>[2x]YSGPKLEDGKVTISFMKELMQWYKDQKKLHRKCAYQILVQVKEVLSKLSTLVETTLKETEKITVCGDTHGQFYD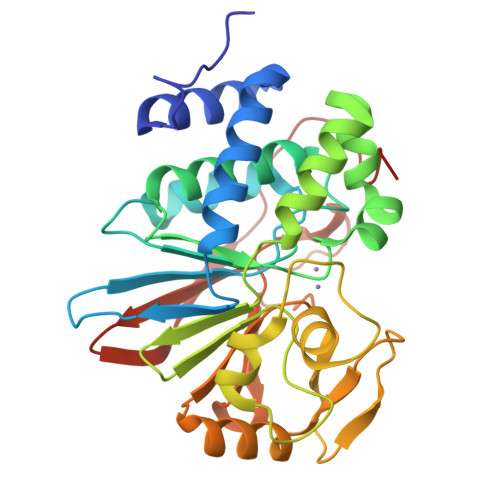LLNIFELNGLPSETNPYIFNGDFVDRGSFSVEVILTLFGFKLLYPDHFHLLRGNHETDNMNQIYGFEGEVKAKYTAQMYELFSEVFEWLPLAQCINGKVLIMHGGLFSEDGVTLDDIRKIERNRQPPDSGPMCDLLWSDPQPQNGRSISKRGVSCQFGPDVTKAFLEENNLDYIIRSHEVKAEGYEVAHGGRCVTVFSAPNYCDQMGNKASYIHLQGSDLRPQFHQFTAVPHPNVKPMAYA>[2x]MRSFPKAKEAFSEGEKVSFGVHRLHVGDAREVLASFPEASVHLVVTSPPYWTLKRYEDTPGQLGHIEDYEAFLDELDRVWREVFRLLVPGGRLVIVVGDVAVARRRFGRHLVFPLHADIQVRCRKLGFDNLNPIIWHKHTNASLEVEGRGVFLGKPYEPGAIIKTEIEYILMQRKPGGYRKPTQEQREKSRLPKEDFHRFFRQIWDDIPGESTKDHPAP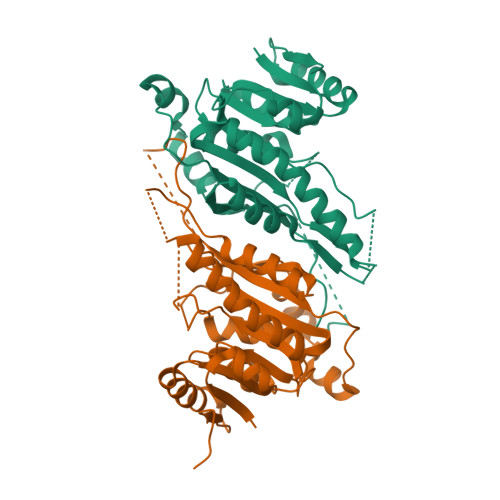FPLELAERLVRMFSFVGDVVLDPFAGTGTTLIAAARWGRRALGVELVPRYAQLAKERFAREVPGFSLEVLDGATHPRR>MKAAAKRISDGVYWTGVLDWDLRNYHGYTLQGTTYNAYLVCGDEGVALIDNSYPGTFDELMARVEDALQQVGMERVDYIIQNHVEKDHSGVLVELHRRFPEAPIYCTEVAVKGLLKHYPSLREAEFMTVKTGDVLDLGGKTLTFLETPLLHWPDSMFTLLDEDGILFSNDAFGQHLCCPQRLDREIPEYILMDAARKFYANLITPLSKLVLKKFDEVKELGLLERIQMIAPSHGQIWTDPMKIIEAYTGWATGMVDERVTVIYDTMHGSTRKMAHAIAEGAMSEGVDVRVYCLHEDDRSEIVKDILESGAIALGAPTIYDEPYPSVGDLLMYLRGL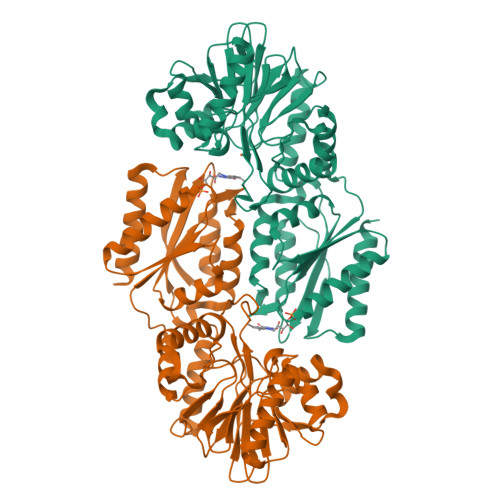KFNRTLTRKALVFGSMGGNGGATGTMKELLAEAGFDVACEEEVYYVPTGDELDACFEAGRKLAAEIRR[8x]> MEPVGCCGECRGSSVDPRSTFVLSNLAEVVERVLTFLPAKALLRVACVCRLWRECVRRVLRTHRSVTWISAGLAEAGHLEGHCLVRVVAEELENVRILPHTVLYMADSETFISLEECRGHKRARKRTSMETALALEKLFPKQCQVLGIVTPGIVVTPMGSGSNRPQEIEIGESGFALLFPQIEGIKIQPFHFIKDPKNLTLERHQLTEVGLLDNPELRVVLVFGYNCCKVGASNYLQQVVSTFSDMNIILAGGQVDNLSSLTSEKNPLDIDASGVVGLSFSGHRIQSATVLLNEDVSDEKTAEAAMQRLKAANIPEHNTIGFMFACVGRGFQYYRAKGNVEADAFRKFFPSVPLFGFFGNGEIGCDRIVTGNFILRKCNEVKDDDLFHSYTTIMALIHLGSSK;>SVFAYESSVHSTNVLLSLNDQRKKDVL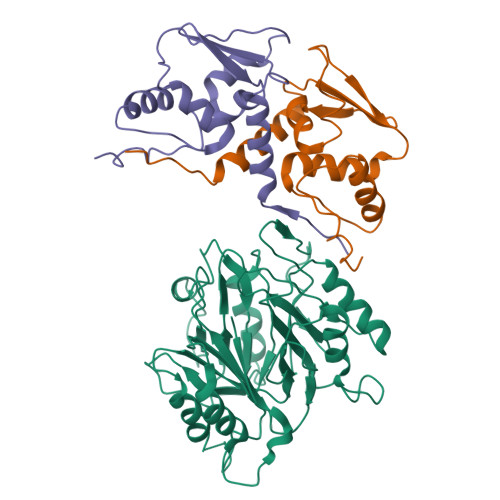CDVTIFVEGQRFRAHRSVLAACSSYFHSRIVGQADGELNITLPEEVTVKGFEPLIQFAYTAKLILSKENVDEVCKCVEFLSVHNIEESCFQFLKF[2x]>GLKLDLTWFDKSTEDFKGEEYSKDFGDDGSVMESLGV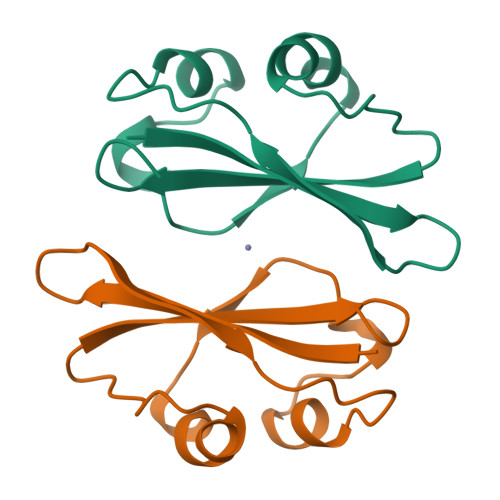PFKDNVNNGCFDVIAEWVPLLQPYFNHQIDISDNEYFVSFDYRDGDW[2x]>MDYRTVFRLDGACAAVTGAGSGIGLEICRAFAASGARLILIDREAAALDRAAQELGAAVAARIVADVTDAEAMTAAAAEAEAVAPVSILVNSAGIARLHDALETDDATWRQVMAVNVDGMFWASRAFGRAMVARGAGAIVNLGSMSGTIVNRPQFASSYMASKGAVHQLTRALAAEWAGRGVRVNALAPGYVATEMTLKMRERPELFETWLDMTPMGR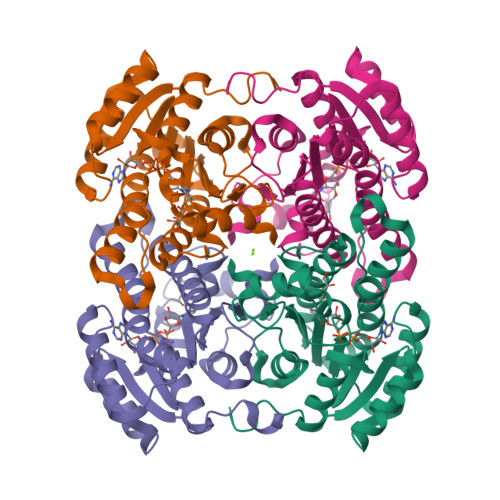CGEPSEIAAAALFLASPAASYVTGAILAVDGGYTVW[4x]>[4x]ATQMRLTDTNLLEVLNSEEYSGVLKEFREQRYSKKAILYTPNTERNLVFLVKSGRVRVYLAYEDKEFTLAILEAGDIFCTHTRAFIQAMEDTTILYTDIRNFQNIVVEFPAFSLNMVKVL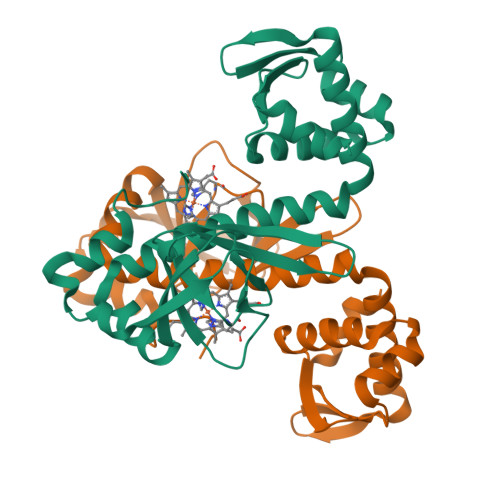GDLLKNSLTIINGLVFKDARLRLAEFLVQAAMDTGLKVPQGIKLELGLNTEEIALMLGTTRQTVSVLLNDFKKMGILERVNQRTLLLKDLQKLKEFSSGV> MVHLGPKKPQARKGSMADVPKELMQQIENFEKIFTVPTETLQAVTKHFISELEKGLSKKGGNIPMIPGWVMDFPTGKESGDFLAIDLGGTNLRVVLVKLGGDRTFDTTQSKYRLPDAMRTTQNPDELWEFIADSLKAFIDEQFPQGISEPIPLGFTFSFPASQNKINEGILQRWTKGFDIPNIENHDVVPMLQKQITKRNIPIEVVALINDTTGTLVASYYTDPETKMGVIFGTGVNGAYYDVCSDIEKLQGKLSDDIPPSAPMAINCEYGSFDNEHVVLPRTKYDITIDEESPRPGQQ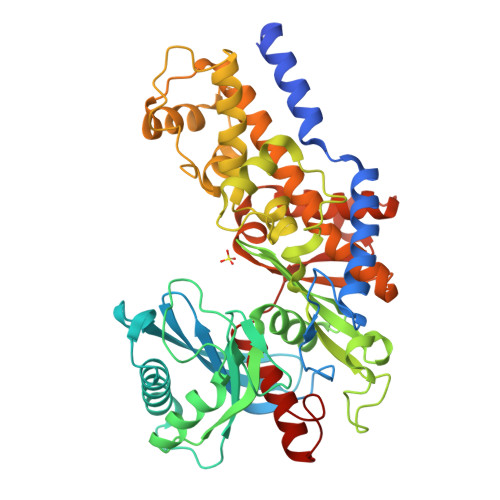TFEKMSSGYYLGEILRLALMDMYKQGFIFKNQDLSKFDKPFVMDTSYPARIEEDPFENLEDTDDLFQNEFGINTTVQERKLIRRLSELIGARAARLSVCGIAAICQKRGYKTGHIAADGSVYNRYPGFKEKAANALKDIYGWTQTSLDDYPIKIVPAEDGSGAGAAVIAALAQKRIAEGKSVGIIGA> SEILNN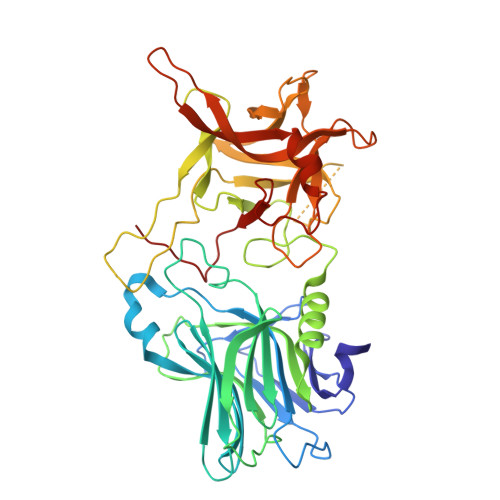IILNLRYKDNNLIDLSGYGAKVEVYDGVELNDKNQFKLTSSANSKIRVTQNQNIIFNSVFLDFSVSFWIRIPKYKNDGIQNYIHNEYTIINCMKNNSGWKISIRGNRIIWTLIDINGKTKSVFFEYNIREDISEYINRWFFVTITNNLNNAKIYINGKLESNTDIKDIREVIANGEIIFKLDGDIDRTQFIWMKYFSIFNTELSQSNIEERYKIQSYSEYLKDFWGNPLMYNKEYYMFNAGNKNSYIKLKKDSPVGEILTRSKYNQNSKYINYRDLYIGEKFIIRRKSNSQSINDDIVRKEDYIYLDFFNLNQEWRVYTYKYFKKEEEKLFLAPISDSDEFYNTIQIKEYDEQPTYSCQLLFKKDEESTDEIGLIGIHRFYESGIVFEEYKDYFCISKWYLKEVKRKPYNLKLGCNWQFIPKDEGWTEPP>MTYRVKIHKQV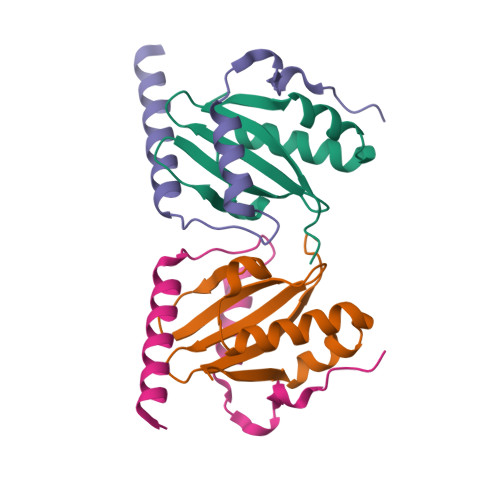VKALQSLPKAHYRRFLEFRDILEYEPVPREKFDVIKLEGTGDLDLYRARLGDYRVIYSVNWKDKVIKILKLKPRGRAYK[2x];>[2x]MRMEKVGDVLKELERLKVEIQRLEAMLMPEERDEDITEEEIAELLELARDEDPENWIDAEELPEPED>[4x]MGLSLPKEKGLILCLWSKFCRWFQRRESWAQSRDEQNLLQQKRIWESPLLLAAKDNDVQALNKLLKYEDCKVHQRGAMGE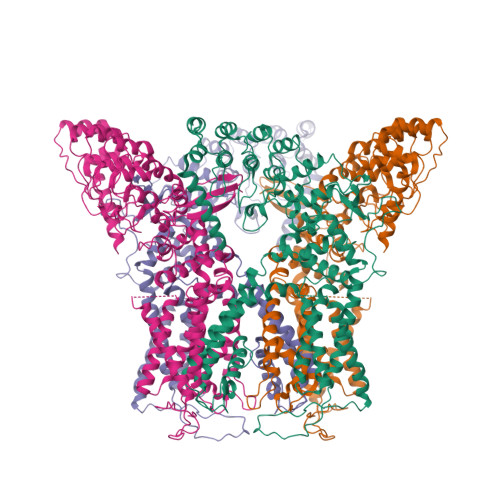TALHIAALYDNLEAAMVLMEAAPELVFEPMTSELYEGQTALHIAVVNQNMNLVRALLARRASVSARATGTAFRRSPCNLIYFGEHPLSFAACVNSEEIVRLLIEHGADIRAQDSLGNTVLHILILQPNKTFACQMYNLLLSYDRHGDHLQPLDLVPNHQGLTPFKLAGVEGNTVMFQHLMQKRKHTQWTYGPLTSTLYDLTEIDSSGDEQSLLELIITTKKREARQILDQTPVKELVSLKWKRYGRPYFCMLGAIYLLYIICFTMCCIYRPLKPRTNNRTSPRDNTLLQQKLLQEAYMTPKDDIRLVGELVTVIGAIIILLVEVPDIFRMGVTRFFGQTILGGPFHVLIITYAFMVLVTMVMRLISASGEVVPMSFALVLGWCNVMYFAEGFQMLGPFTIMIQKMIFGDLMRFCWLMAVVILGFASAFYIIFQTEDPEELGHFYDYPMALFSTFELFLTIIDGPANYNVDLPFMYSITYAAFAIIATLLMLNLLIAMMGDTHWRVAHERDELWRAQIVATTVMLERKLPRCLWPRSGICGREYGLGDRWFLRVEDRQDLNRQRIQRYAQAFHTRGSEDLDKDSVEKLELGCPFSPHLSLPMPSVSRSTSRSSANWERLRQGTLRRDLRGIINRGLEDGESWEYQILVPRGSAAAWSHPQFEK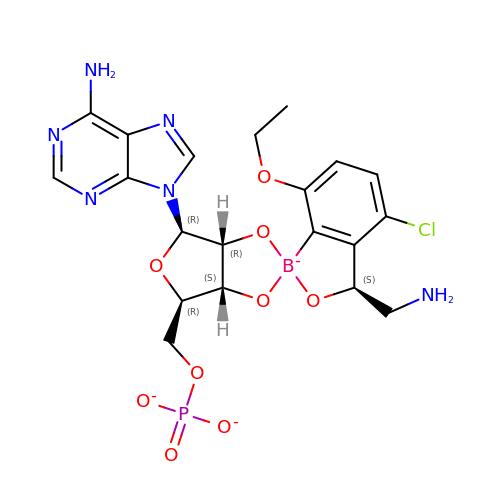4-Chloro-3-aminomethyl-7-[ethoxy]-3H-benzo[C][1,2]oxaborol-1-ol modified adenosine | C20 H22 B Cl N6 O9 P | QVHGEDIRODVXDV-RIMGRJFKSA-L> MERAEILGVGTELLYGETLDTNTAEIARSLKPYALKVERTLRVADEVAPLAREVEEAFARARLVVLSGGLGPTPDDVTREAVALALGEPLELDEAVLGEIEAFFRARGRAMPEANRKQAMRIPSATWLKNPRGTAPGWWVRKGGKDLVLLPGPPPEWRPMWQEVLPRLGLPRRPYAERVLKTWGIGESEIVERLGPLFVREEEEEVGTYPKVHGVEVVVRGREDRVAELAERIKKKLLKEVWGEGEMTLAEAVKRR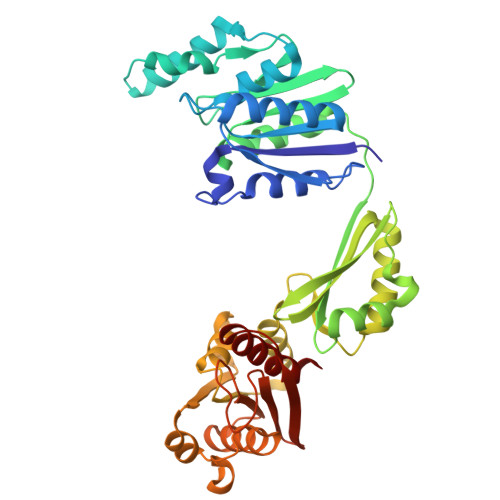MEREGATLSTMESLTGGLLGAEITRVPGASRFYLGGVVSYSVGAKARFGVPQDLLSRTVSAETARAMAEAARSLFGSTYALATTGVAGPDPLEGEPPGTVYVALAGPTGAEVRRYRFPGDRETVRLRSVYAALALLVT>[2x]GNVGKISLDQIDLLSTKSFPPCMRQLHKALRENHHLRHGGRMQYG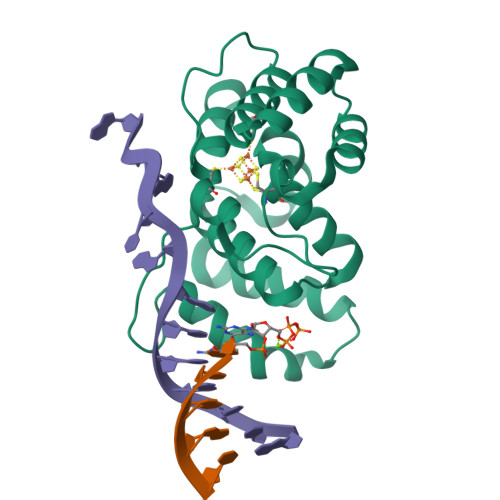LFLKGIGLTLEQALQFWKQEFIKGKMDPDKFDKGYSYNIRHSFGKEGKRTDYTPFSCLKIILSNPPSQGDYHGCPFRHSDPELLKQKLQSYKISPGGISQILDLVKGTHYQVACQKYFEMIHNVDDCGFSLNHPNQFFCESQRILN>[4x]SMNFYSAYQHGFVRVAACTHHTTIGDPAA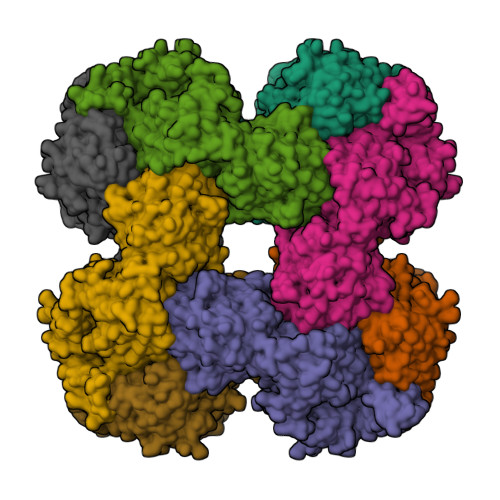NAASVLDMARACHDDGAALAVFPELTLSGYSIEDVLLQDSLLDAVEDALLDLVTESADLLPVLVVGAPLRHRHRIYNTAVVIHRGAVLGVVPKSYLPTYREFYERRQMAPGDGERGTIRIGGADVAFGTDLLFAASDLPGFVLHVEICEDMFVPMPPSAEAALAGATVLANLSGSPITIGRAEDRRLLARSASARCLAAYVYAAAGEGESTTDLAWDGQTMIWENGALLAESERFPKGVRRSVADVDTELLRSERLRMGTFDDNRRHHRELTESFRRIDFALDPPAGDIGLLREVERFPFVPADPQRLQQDCYEAYNIQVSGLEQRLRALDYPKVVIGVSGGLDSTHALIVATHAMDREGRPRSDILAFALPGFATGEHTKNNAIKLARALGVTFSEIDIGDTARLMLHTIGHPYSVGEKVYDVTFENVQAGLRTDYLFRIANQRGGIVLGTGDLSELALGWSTYGVGDQMSHYNVNAGVPKTLIQHLIRWVISAGEFGEKVGEVLQSVLDTEITPELIPTGEEELQSSEAKVGPFALQDFSLFQVLRYGFRPSKIAFLAWHAWNDAERGNWPPGFPKSERPSYSLAEIRHWLQIFVQRFYSFSQFKRSALPNGPKVSHGGALSPRGDWRAPSDMSARIWLDQIDREVPKG>MLGSSSLSIRTTDDKSLFARTMDFTMEPDSKVIIVPRNYGIRLLEKENVVINNSYAFVGMGSTDITSPVLYDGVNEKGLMGAMLYYATFATYADEPKKGTRGINPVYVISQVLGNCVTVDDVIEKLTSYTLLNEANIILGFAPPLHYTFTDASGESIVIEPDKTGITIHRKTIGVMTNSPGYEWHQTNLRAYIGVTPNPPQDIMMGDLDLTPFGQGAGGLGLPGDFTPSARFLRVAYWKKYTEKAKNETEGVTNLFHILSSVNIPKGVVLTNEGKTDYTIYTSAMCAQSKNYYFKLYDNSRISAVSLMAENLNSQDLITF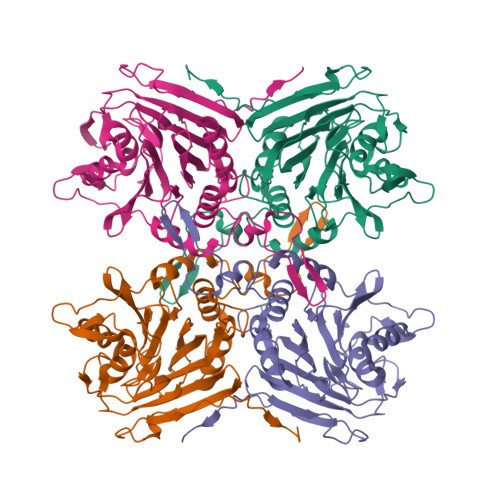EWDRKQDIKQLNQVNVMS[4x]>[2x]RSPWGDELLNICMNAKHHKRVPSPEDKLYEECIPWKDNACCTLTTSWEAHLDVSPLYNFS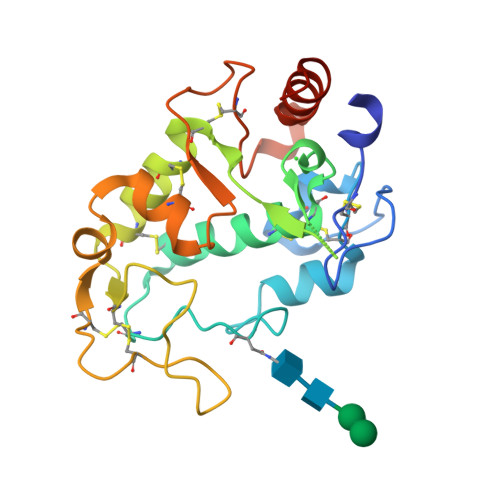LFHCGLLMPGCRKHFIQAICFYECSPNLGPWIQPVGSLGWEVAPSGQGERVVNVPLCQEDCEEWWEDCRMSYTCKSNWRGGWDWSQGKNRCPKGAQCLPFSHYFPTPADLCEKTWSNSFKASPERRNSGRCLQKWFEPAQGNPNVAVARLFASEFLEVLFQ In archaea, the adaptor protein CheF resides at the cytoplasmic face of the archaeal C-ring formed by the proteins ArlCDE and interacts with phosphorylated CheY. In archaea, CheY-P binds to CheF, an adaptor protein uniquely present in archaeal species, however the precise mechanism of this interaction is unclear to date. Binding of CheY-P to CheF induces a rotational switch of the archaellum. CheF forms a twisted homodimer offering two CheY-P binding sites within an elongated C-terminal tail domain.

However, we could successfully use the dataset deposited by Paithankar and coworkers, to solve the structure of the P. horikoshii at 2.75 Å by molecular replacement (MR) using our initial MjCheF model and obtained a complete model of CheF. CheF consists of two N-terminal domains and a long C-terminal tail that reaches out from the center of the two domains and extends into a long tail domain of over ~80 Å in length. The first N-terminal domain is formed by seven β-strands (i.e., β1-β7) and an α-helix and connecting it to the second domain. This second N-terminal domain consists of eight β-strands (i.e., β8-β15) and is connected to a small helical bundle (i.e., α2-α4) central to the two N-terminal domains. Helix α4 spans into an elongated C-terminal domain (CTD) that is formed by α5-α7, a long β-strand (i.e., β16) and the C-terminal helix α8. The asymmetric unit contained two CheF molecules, which interacted through their C-termini employing a buried surface area of 2700 A2. The strongest determinant of this interface is a substantial β-sheet, jointly being formed by the β16 strands of each of the CheF monomers. Moreover, both monomers of the CheF homodimer do not align symmetrically to each other but instead tilt their N-terminal domains by 90°. The residues involved in bending are E265 to L267 within helix α8 (obtained from DynDom47). This observation suggests that the CheF homodimer exhibits an intrinsic flexibility with respect to its N-terminal domains, which might be of functional relevance. Thus, our crystal structure suggests a CheF homodimer, which was confirmed in solution by mass photometry (MP).

>[2x]PIFEARVKVGISSSWVTSRKVSWRDAIAQIESDRIVVKYLKMGEVVGEDSFPFSALIDLGVRIPDELKLNPEKDHFGIKFYIPGRGELLVIFTIEENLLIYDEKKFSEFVHKVFEVLINGKTVMLQLARIIGGAVNMESKWEEGWLRVIKVKSARTQKTERSIVVIIKDKRPVSIFSDLEDIEIEEVDMNGKRVRAWKIRHFHIDQSVTSYLYIPDKQTQLYVLRYLLKYNPAIMEFIMKVSDDFPTLKSEFQEIMEKEIKELEALDEMEKQILVALYSGINPLELHQFLGVSEKEIEEIYDRMIDKGLLKIVMIRKIVDLTNEGRKIVNKLLKYGLVSM N-{(1S)-2-(dimethylamino)-2-oxo-1-[3-(trifluoromethyl)phenyl]ethyl}-4'-(trifluoromethyl)[1,1'-biphenyl]-2-carboxamide | C25 H20 F6 N2 O2 | 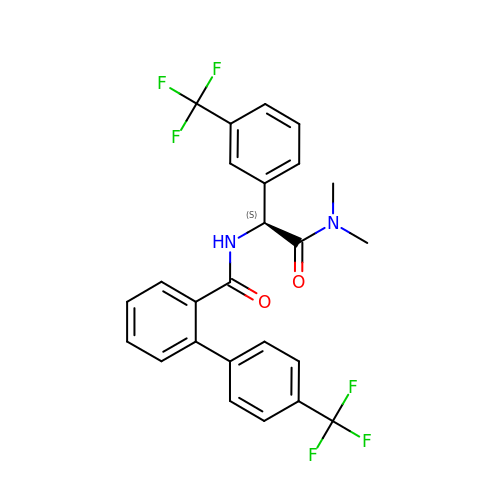XHKLRVAMXWYKMX-NRFANRHFSA-N[1-(6-chloropyrimidin-4-yl)-1H-pyrazol-4-yl]boronic acid | C7 H6 B Cl N4 O2 | 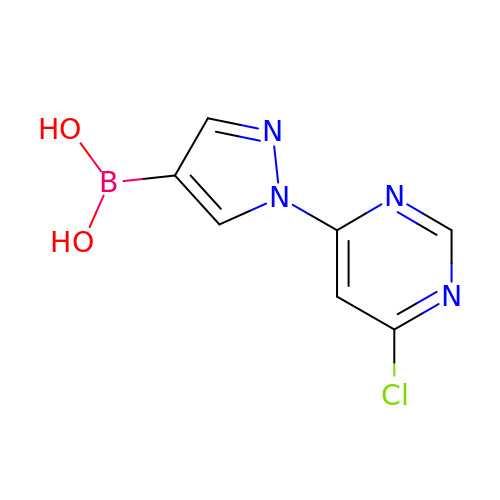FINXKFQNFLSJBL-UHFFFAOYSA-N>GHMPTKQQLLYEGKAKKIYATDEPDVLWVEYKDSATAFNGEKKATIAGKGRLNNEISSLLFLKLREAGIANHFIEKLSPTEQLVRRVTIIPLEVVVRNVVAGSLAKRIGLEEGTPLEAPLVEFYYKNDDLGDPLLLEDHIFILKLASREEVAALKQAALAVNDVLRLHFAERNVRLIDFKLEFGRTADGAILLADEISPDTCRLWDAKTNEKLDKDVF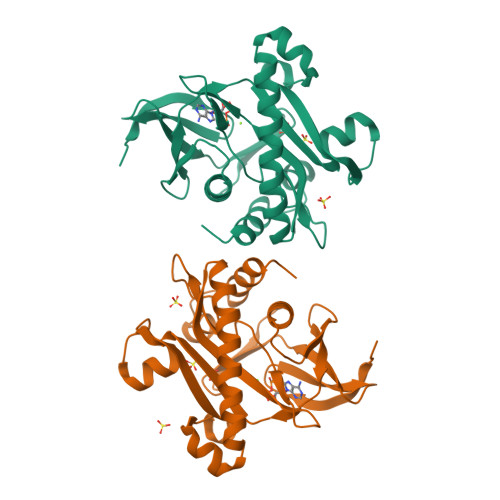RRDLGSLTDAYEVILQRLGGESACTK[2x]>[2x]MHHHHHHTSKIEQPRWASK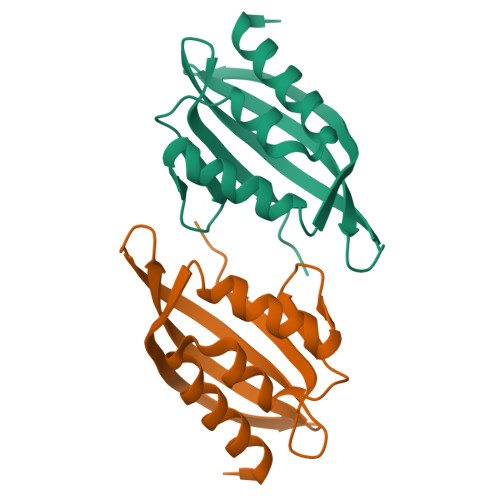DDAAGKASTPDEKIVLEFMDALTSNDAAKLIDYFAEDTMYQNMPLPPAYGRDAVEQTLAGFFKVFSIDAVETFHIGSTKGLVYTERVDVLRALPTGKSYNVSVLGVFQLTEGKITGWRDYFDLREVEEAVDLPFRG> MGSSHHHHHHSQDPMMDVLVSECSARLLQQEEEIKSLTAEIDRLKNCGCLGASPNLEQLQEENLKLKYRLNILRKSLQAERNKPTKNMINIISRLQEVFGHAIKAAYPDLENPPLLVTPSQQAKFGDYQCNSAMGISQMLKTKEQKVNPREIAENITKHLPDNECIEKVEIAGPGFINVHLRKDFVSEQLTSLLVNGVQLPALGENKKVIVDFSSPNIAKEMHVGHLRSTIIGESISRLFEFAGYDVLRLNHVGDWGTQFGMLIAHLQDKFPDYLTVSPPIGDLQVFYKESKKRFDTEEEFKKRAYQCVVLLQGKNPDITKAWKLICDVSRQELNKIYDALDVSL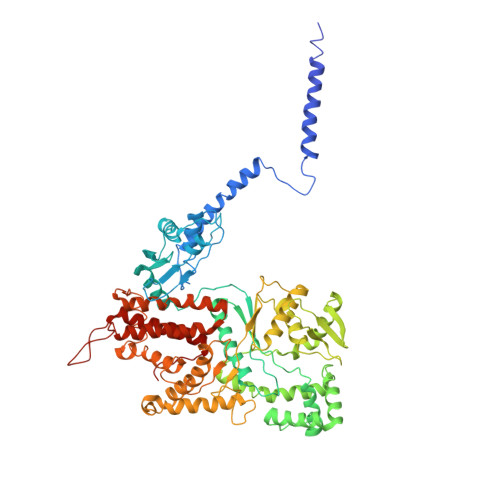IERGESFYQDRMNDIVKEFEDRGFVQVDDGRKIVFVPGCSIPLTIVKSDGGYTYDTSDLAAIKQRLFEEKADMIIYVVDNGQSVHFQTIFAAAQMIGWYDPKVTRVFHAGFGVVLGEDKKKFKTRSGETVRLMDLLGEGLKRSMDKLKEKERDKVLTAEELNAAQTSVAYGCIKYADLSHNRLNDYIFSFDKMLDDRGNTAAYLLYAFTRIRSIARLANIDEEMLQKAARETKILLDHEKEWKLGRCILRFPEILQKILDDLFLHTLCDYIYELATAFTEFYDSCYCVEKDRQTGKILKVNMWRMLLCEAVAAVMAKGFDILGIKPVQRM> LQYTSSARQALRATALVLNFFPLGYTCGPKNKQ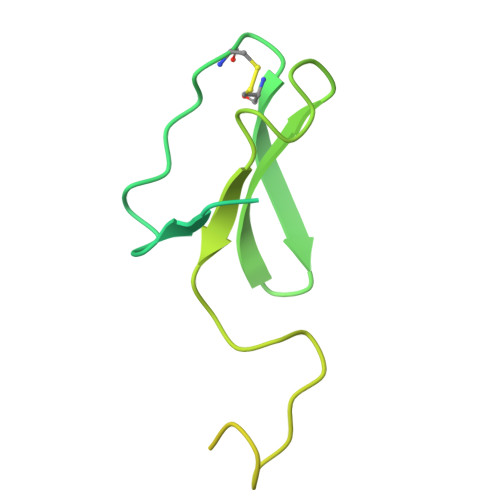VFFPPNNLDGRTTHQMKKLQGSTDKHPGLVPRDKLKLHCEFCRFHWVQDTLVVRCAAHPKEHNQREIWLEPTWTWGKQQPYQYYKYMPVNINPRTGMPLAREDAKGMNNERRSQGLPTKTRLLERERRGISRAITGLGIYNQRWQTRFPFAT>[2x]MGHHHHHHMVKDQAEQLRLKLSRLRQQPSPRTIAVTSGKGGVGKSNVSLNFSLSLSKLGFRVLLLDMAIGMGNIDILLGESSSLALADWFSARLPLSELVKSGPEHLSYIAGGTGAAQWQGLDTASIDRFLTELQAVASQYDYLIFDMGAGASGERLYFLKSVDDVFVVTTPEPTAMTDAYAMMKYMHAAGSEAPFSVIVNRAGKEREGYEVFERLKHVT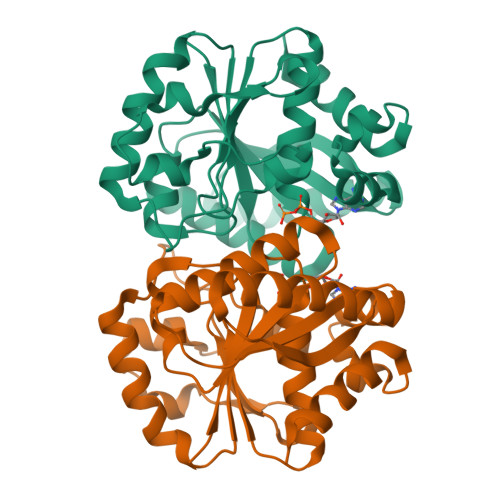GRFLNKDIALLGIIPEDRTVARAVVSQTPFVLLDPAAKASKAVRQMAFRYAPQREEGTERASRFFAKLRQLFLER>MQFSKMHGLGNDFMVVDAVTQNVFFSPELIRRLADRHLGVGFDQLLVVEPPYDPELDFHYRIFNADGSEVAQCGNGARCFARFVRLKGLTNKRDIRVSTANGRMVLTVTDDDLVRVNMGEPNFEPSAVPFRANKAEKTYIMRAAEQTILCGVVSMGNPHCVIQVDDVDTAAVETLGPVLESHERFPERANIGFMQVVKREHIRLRVYERGAGETQACGSGACAAVAVGIQQGLLAEEVRVELPGGRLDIAWKGPGHPLYMTGPAVHVADGFIHLH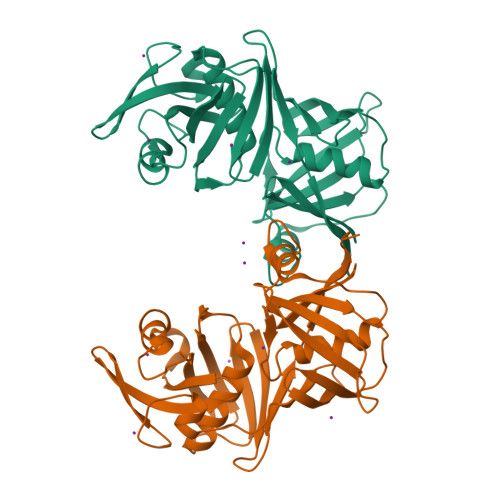HHHHH[2x]> GAAEKTVVNISKVDGMPWFNRMGEGVVQAGKEFNLNASQVGPSSTDAPQQVKIIEDLIARKVDAITIVPNDANVLEPVFKKARDAGIV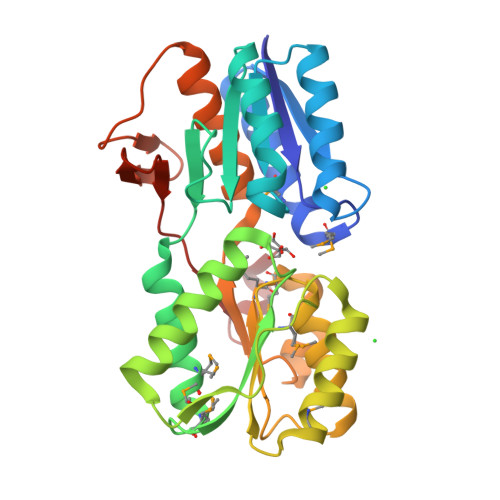VLTNESPGQPSANWDVEIIDNEKFAAEYVEHMAKRMGGKGGYVIYVGSLTVPQHNLWADLLVKYQKEHYPDMHEVTRRMPVAESVDDSRRTTLDLMKTYPDLKAVVSFGSNGPIGAGRAVKEKRAKNKVAVYGMMIPSQAASLIKSGDITEGITYDPATAGYALAAVASTLLNGKTIEPGFELKELGKAEVDSDKHIIRFHKVLLVNKDNIDSLY>MPLPPDITFDSLALIKMHSQNMKRILEVTLAKFTV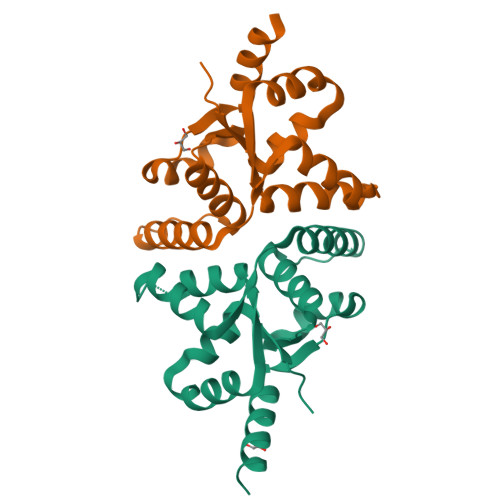NLSIVTVYRYLTARAYLKKNIEAEFEILKDIYNIVPLLDDIAIKAAQIEANLIKKEITLDMEDIITATTAIYTNSLLVTDDPKRYEPIRRFGLDTMPLDKFIKEVELMVEKELI[2x]>[2x]MAKP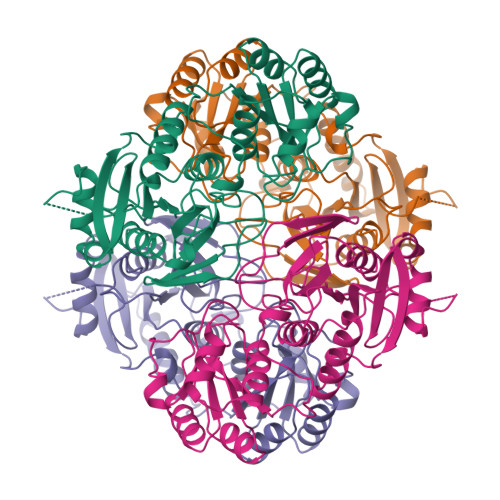QVTILATGGTIAGSGESSVKSSYSAGAVTVDKLLAAVPAINDLATIKGEQISSIGSQEMTGKVWLKLAKRVNELLAQKETEAVIITHGTDTMEETAFFLNLTVKSQKPVVLVGAMRPGSSMSADGPMNLYNAVNVAINKASTNKGVVIVMNDEIHAAREATKLNTTAVNAFASPNTGKIGTVYYGKVEYFTQSVRPHTLASEFDISKIEELPRVDILYAHPDDTDVLVNAALQAGAKGIIHAGMGNGNPFPLTQNALEKAAKSGVVVARSSRVGSGSTTQEAEVDDKKLGFVATESLNPQKARVLLMLALTKTSDREAIQKIFSTY>[2x]GSMSNMDIDGINTGTIDKTPEEITSGTSGTTRPIIRPATLAPPSNKRTRNPSPERATTSSEDDVGRKTQKKQTPTEIKKSVYNMVVKLGEFYNQMMVKAGLNDDMERNLIQNAHAVERILLAATDDKKTEFQKKKNARDVKEGKEEIDHNKTGGTFYKMVRDDKTIYFSPIRITFLKEEVKTMYKTTMGSDGFSGLNHIMIGHSQMNDVCFQRSKALKRVGLDPSLISTFAGSTIPRRSGATGVAIKGGGTLVAEAIRFIGRAMADRGLLRDIKAKTAYEKIL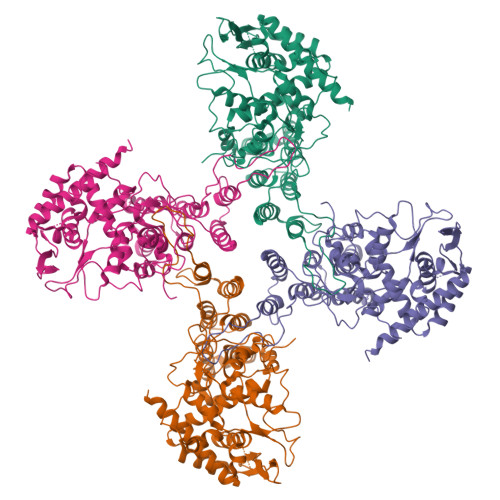LNLKNKCSAPQQKALVDQVIGSRNPGIADIEDLTLLARSMVVVRPSVASKVVLPISIYAKIPQLGFNVEEYSMVGYEAMALYNMATPVSILRMGDDAKDKSQLFFMSCFGAAYEDLRVLSALTGTEFKPRSALKCKGFHVPAKEQVEGMGAALMSIKLQFWAPMTRSGGNEVGGDGGSGQISCSPVFAVERPIALSKQAVRRMLSMNIEGRDADVKGNLLKMMNDSMAKKTSGNAFIGKKMFQISDKNKTNPVEIQIKQTIPNFFFGRDTAEDYDDLDY>MKQYLELMQKVLDEGTQKNDRTGTGTLSIFGHQMRFNLQDGFPLVTTKRCHLRSIIHQLLWFLQGDTNIAYLHENNVTIWDEWADENGDLGPVYGKQWRAWPTPDGRHIDQITTVLNQLKNDPDSRRIIVSAWNVGELDKMALAPCHAFFQFYVADGKLSCQLYQRSCDVFLGLPFNIASYALLVHMMAQQCDLEVGDFVWTGGDTHLYSNHMDQTHLQLSREPRPLPKLIIKRKPESIFDYRFEDFEIEGYDPHPGIKAPV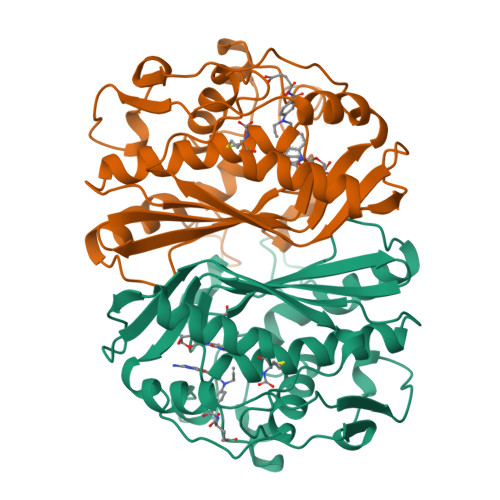AI[2x]> MRNAIFPRIDFLRYLKKIHVSYCPTRPKTEIAKQLIMRVTSES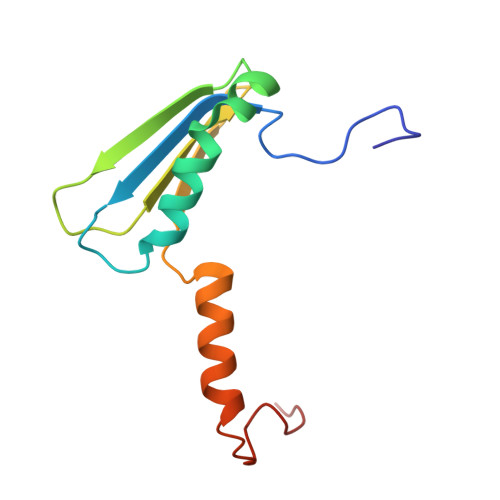VKKKFPHLQASWEMLAYDAPATVEVELLDGRRVRRIIDGYSKAEKKKIVDDWRFTANMEPWPEVLGPQP>[2x]MSGSPAPQGALRQRIVASTPKKTKESKDGAASDAELDKLVKEAAAAKAPAGSERDYKIAFAIITALAFLTRFWGISHPDQVVFDEVHFGKFASYYLQRTYFFDVH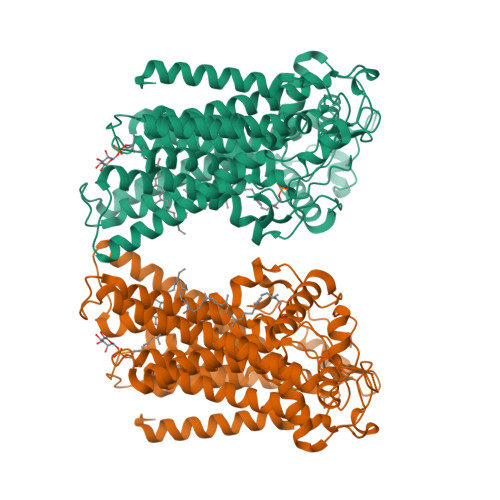PPLGKLLFAFMGWLVGYDGHFHFDNIGDPYVINKVPYVAFRALPAILGSLTVSVVFLIMWESGYSLPACILASGLVLLDNAHIGQTRLILLDATLVFAMACSLLCYIKFYKLRHEPFSRKWWKWLILTGFALSCDISTKYVGLFAFITIGSAVCIDLWDLLNINRPKGALTLPQFGKHFAARAFGLIFMPFMFYLFWFQVHFSILTRSGPGDDFMTPEFQETLSDNIMLANAVTIDYWDTITIKHKETKAYLHSHPDRYPLRYDDGRVSSQGQQVTGYPFNDTNNWWQILPAGPFEEPKLGRHVKHRDLVRLRHVGTDTYLLSHDVASPYYPTNQEFTTVSFNEAYGDRAADTLFEVRIEHGKPGQEFKSISSHFKLIHNPSKVAMWTHPTPLPDWGHRQQEINGNKQIAPSSNVWLVEDIVSLPADHKRREKPERKVKTLPFLRKWFELQRSMFWHNNQLTASHPYASLPYQWPFLLRGVSFWTNSETRQQIYFLGNPVGWWIASSVLAIYVGIVLADQFSLRRGIDALDHRTRSRLYNSTGFFFLAWATHYFPFFVMGRQLFLHHYLPAHLASTLVTGALVEFIFSPEAPEHEIAAQQAKSSSSGKRGGVAMKRHITARERFAGQSLMGSWIATAVILALVAWSWWFFLPLTYGYPGMSVQQVLRRKWLGYDLHFAKLEVLFQGPGSHHHHHHHHHH>GHMSGGGEQADILPANYVVKDRWKVLKKIGGGGFGEIYEAMDLLTRENVALKVE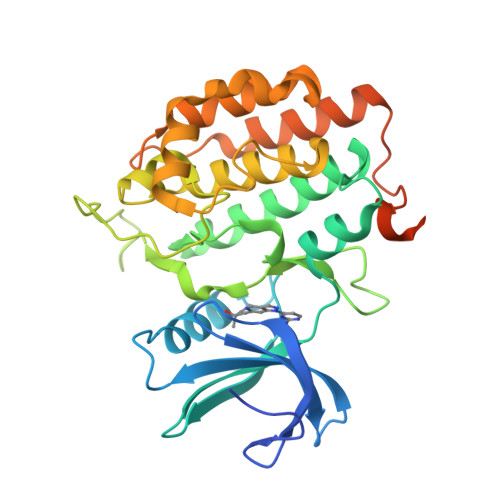SAQQPKQVLKMEVAVLKKLQGKDHVCRFIGCGRNEKFNYVVMQLQGRNLADLRRSQPRGTFTLSTTLRLGKQILESIEAIHSVGFLHRDIKPSNFAMGRLPSTYRKCYMLDFGLARQYTNTTGDVRPPRNVAGFRGTVRYASVNAHKNREMGRHDDLWSLFYMLVEFAVGQLPWRKIKDKEQVGMIKEKYEHRMLLKHMPSEFHLFLDHIASLDYFTKPDYQLIMSVFENSMKERGIAENEAFDWEKAGTDALLSTSTSTPPQQNTRQTAAMFGVVNV[2x]> IIGGQDAAHGAWPWMVSLQIFTYHNNRRYHVCGGSLLNSQWLLTAAHCFRIKKKVTDWRLIFGAKEVEWGTNKPVKPPLQERYVEKIIIHEKYSASSEANDIALMKITPPVTCGHFIGPGCLPQFRAGPPRVPQTCWVAGWGFLQENARRTSP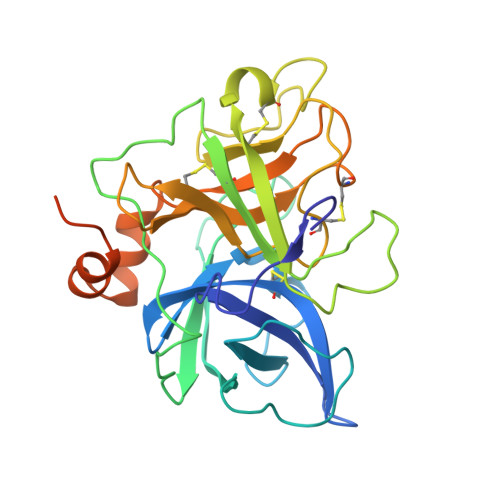MLQEARVDLIDLGLCNSTRWYNGRIRSTNVCAGYPEGKIDTCQGDSGGPLMCKDSAENSYVVVGITSWGVGCARAKRPGVYTSTWSYLNWIASKIGSTAVHMIQLPTASPASTPGAQASSGSVQPSVRPPWFFQQIT> GSMALFSAQSPYINPIIPFTGPIQGGLQEGLQVTLQGTTKSFAQRFVVNFQNSFNGNDIAFHFNPRFEEGGYVVCNTKQNGQWGPEERKMQMPF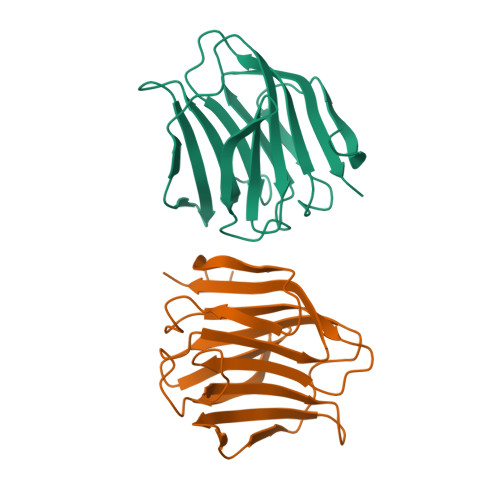QKGMPFELCFLVQRSEFKVMVNKKFFVQYQHRVPYHLVDTIAVSGCLKLSFITFQTQNFRPAHQA>[5x]GQDMVSPPPPIADEPLTVNTGIYLIESYS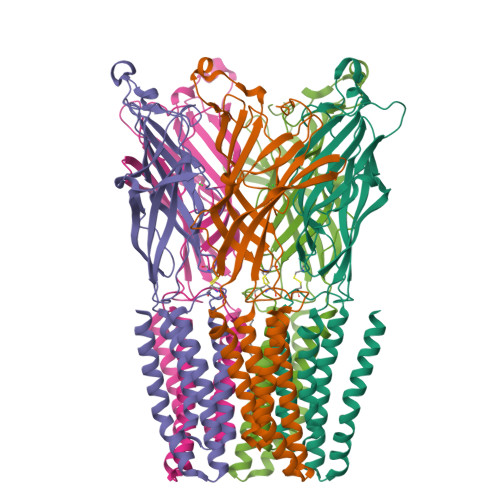LDDCAETFKVNAFLSLSWKDRRLAFDPVRSGVRVKTYEPEAIWIPEIRFVNVENARDADVVDISVSPDGTVQYLERFSARVLSPLDFRRYPFDSQTLHIYLIVRSVDTRNIVLAVDLEKVGKNDDVFLTGWDIESFTAVVKPANFALEDRLESKLDYQLRISRQYFSYIPNIILPMLFILFISWTAFWSTSYEANVTLVVSTLIAHIAFNILVETNCPKTPYMTYTGAIIFMIYLFYFVAVIEVTVQHYLKVESQPARAASITRASRIAFPVVFLLANIILAFLFFGF> WSHPQFEKGSQGGLSQDFVEALKAVVGSPHVSTASAVREQHGHDESMHRCQPPDAVVWPQNVDQVSRVASLCYNQGVPIIPFGTGTGVEGGVCAVQGGVCINLTHMDQITELNTEDFSVVVEPGVTRKALNTHLRDSGLWFPVDPGADASLCGMAATGASGTNAVRYGTMRDNVINLEVVLPDGRLLHTAGRGRHYRKSAAGYNLTGLFVGSEGTLGIITSTTLRLHPAPEATVAATCAFPSVQAAVDSTVQILQAAVPVARIEFLDDVMMDACNRHSKLNCPVAPTLFLEFHGSQQTLAEQLQRTEAITQDNGGSHFSWAKEAEKRNELWAARHNAWYAALALSPGSKAYSTDVCVPISRLPEILVETKEEIKASKLTGAIVGHVGDGNFHCILLVDPDDAEEQRRVKAFAENLGRRALALGGTCTGEHGIGLGKRQLLQEEVGPVGVETMRQLKNTLDPRGLMNPGKVL

Mammalian lactate dehydrogenase D (LDHD) catalyzes the oxidation of D-lactate to pyruvate. We demonstrate that mLDHD is an Mn2+-dependent general dehydrogenase which exhibits catalytic activity for D-lactate and other D-2-hydroxyacids containing hydrophobic moieties, but no activity for their L-isomers or D-2-hydroxyacids containing hydrophilic moieties. Similar to other members of the VAO/PCMH flavoprotein family, mLDHD consists of an FAD-binding domain, a substrate-binding domain and a C-terminal domain. The substrate-binding site contains a positively charged pocket to bind the common glycolate moiety and a hydrophobic pocket with some elasticity to bind the varied hydrophobic moieties of substrates.

To elucidate the molecular basis for the substrate preference and catalytic reaction of mLDHD, we determined the crystal structure of wild-type (WT) mLDHD in FAD-bound form (mLDHDFAD, 1.70 Å resolution) and in complex with FAD, Mn2+, and D-lactate (mLDHDFAD+Mn+D-LAC, 1.73 Å resolution). There is a non-covalently bound FAD at the active site, which is apparently derived from the expression system, indicating that FAD binds to mLDHD tightly. In the WT mLDHDFAD and mLDHDH405AFAD structures, there is no density for metal ion and ligand at the active site. Later structure determination of mLDHD in FAD-bound form confirms that there is no metal ion bound at the active site (see discussion later). In the mLDHDFAD structure, the substrate-binding site is occupied by a water molecule. Comparison of the mLDHDFAD and mLDHDFAD+Mn+D-LAC structures shows that the binding of Mn2+ and D-lactate causes only very subtle conformational changes of a few residues composing subsite A including His398, His405, and Glu442, which rotate their side chains slightly to better coordinate Mn2+. Comparison of the mLDHDFAD and mLDHDH405AFAD structures reveals no notable conformational differences at the active site.>RSPWEENFSRSYPCDEKKQNDSVIAECSNRRLQEVPQTVGKYVTELDLSDNFITHITNESFQGLQNLTKINLNHNPNVQHQNGNPGIQSNGLNITDGAFLNLKNLRELLLEDNQLPQIPSGLPESLTELSLIQNNIYNITKEGISRLINLKNLYLAWNCYFNKVCEKTNIEDGVFETLTNLELLSLSFNSLSHVPPKLPSSLRKLFLSNTQIKYISEEDFKGLINLTLLDLSGNCPRCFNAPFPCVPCDGGASINIDRFAFQNLTQLRYLNLSSTSLRKINAAWFKNMPHLKVLDLEFNYLVGEIASGAFLTMLPRLEILDLSFNYIKGSYPQHINISRNFSKLLSLRALHLRGYVFQELREDDFQPLMQLPNLSTINLGINFIKQIDFKLFQNFSNLEIIYLSENRISPLVKDTRQSYANSSSFQRHIRKRRSTDFEFDPHSNFYHFTRPLIKPQCAAYGKALDLSLNSIFFIGPNQFENLPDIACLNLSANSNAQVLSGTEFSAIPHVKYLDLTNNRLDFDNASALTELSDLEVLDLSYNSHYFRIAGVTHHLEFIQNFTNLKVLNLSHNNIYTLTDKYNLESKSLVELVFSGNRLDILWNDDDNRYISIFKGLKNLTRLDLSLNRLKHIPNEAFLNLPASLTELHINDNMLKFFNWTLLQQFPRLELLDLRGNKLL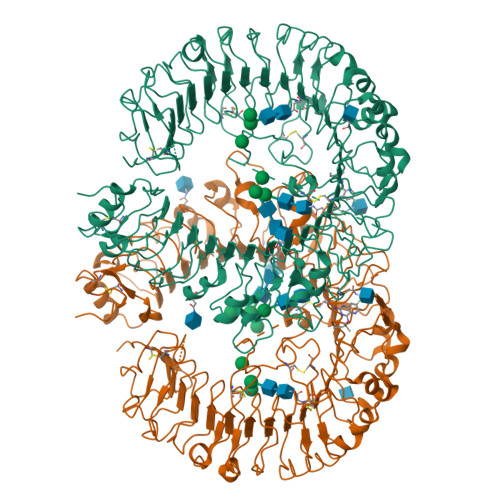FLTDSLSDFTSSLRTLLLSHNRISHLPSGFLSEVSSLKHLDLSSNLLKTINKSALETKTTTKLSMLELHGNPFECTCDIGDFRRWMDEHLNVKIPRLVDVICASPGDQRGKSIVSLELTTCVSDVTEFLVPR[4x]> GHMSTFLPAPLQCGRFELTFERPLVMGILNATPDSFSDGGRFLARDDALRRAERMIAEGADLLDIGGESTRPGAPPVPLDEELARVIPLVEALRPLNVPLSIDTYKPAVMRAALAAGADLINDIWGFRQPGAIDAVRDGNSGL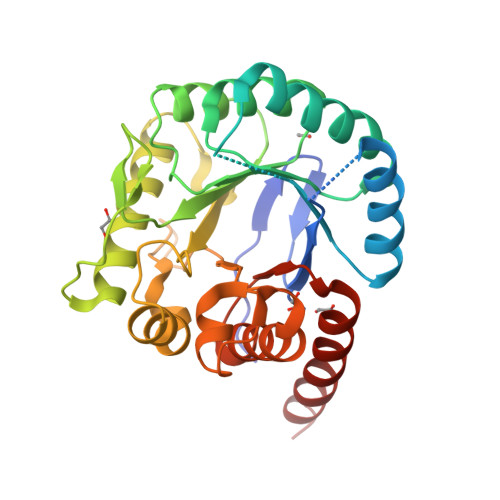CAMHMLGEPQTMQVGEPDYGDVVTDVRDFLAARAQALRDAGVAAERICVDPGFGFGKAVVDDNYALLAALPDTAPARPDGRAYPILAGMSRKSMLGAVIGGKPPLERVAASVAAALCAVERGAAIVRVHDVAATVDALSVWNAVRAAARQR> 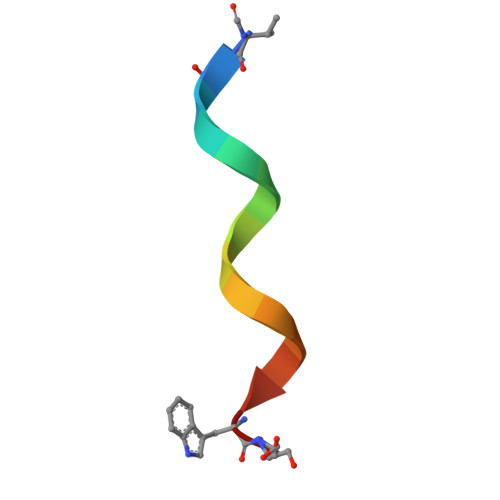VGALAVVVWLWLWLWX>HHHHHHMTTINPTNYTLLKKQAASLIEDEHHMIAILSNMSALLNDN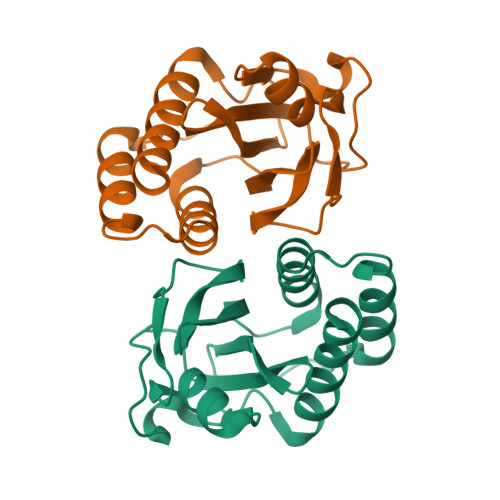LDQINWVGFYLLEQNELILGPFQGHPACVHIPIGKGVCGTAVSERRTQVVADVHQFKGHIACDANSKSEIVVPIFKDDKIIGVLDIDAPITDRFDDNDKEHLEAIVKIIEKQLA[8x]> PTHITIGIYFKP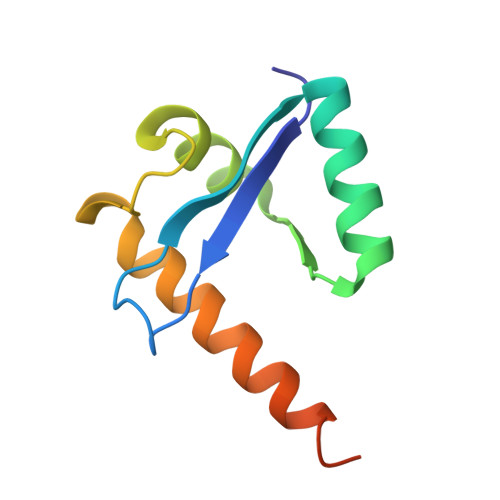ELMPIPMISVYETNQRALAVRAYAEKVGVPVIVDIKLARSLFKTHRRYDLVSLEEIDEVLRLLVWLEEVENAGKDVIQPQENEVRH> MFNQFNPLVYTHGGKLERKSKKDKTASKVFEEFGVMEAYNCWKEASLCIQQRDKDSVLKLVAALNTYKDAVEPIFDSRLNSAQEVLQPSILEEFFEYLFSRIDSIVGVNIPIRHPAKGYLSLSFNPHNIETLIQSPEYTVRAKDHDFIIGGSAKLTIQGHGGEGETTNIVVPAVAIECK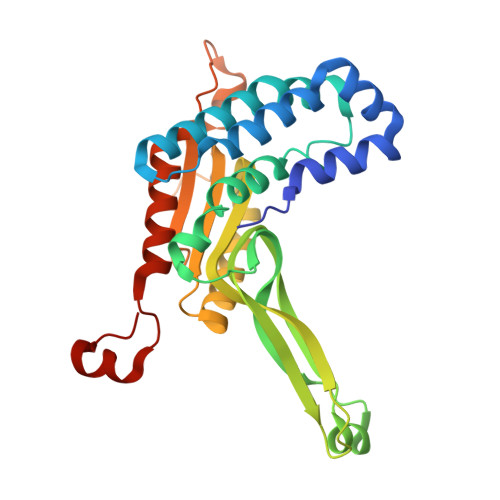RYLERNMLDECAGTAERLKRATPYCLYFVVAEYLKLDDGAPELTEIDEIYILRHQRNSERNKPGFKPNPIDGELIWDLYQEVMNHLGKIWWDPNSALQRGKVFNRP> LQIYPQRRVIGHRIEIFRGKHRRRRMVPPRIPLHPLAANTSEETASKDMNLFETYRDLQLRWKKTCRQRKKKFNIARKWRMPRNIRPLPDPSWTLVFHVNPRSGYRRGRGVCRDRRRENLQGDALEVSAEDEENRLAGKAPSNRDQEDRQRGRGAQETYFRSGAALDAAIEEENILQIL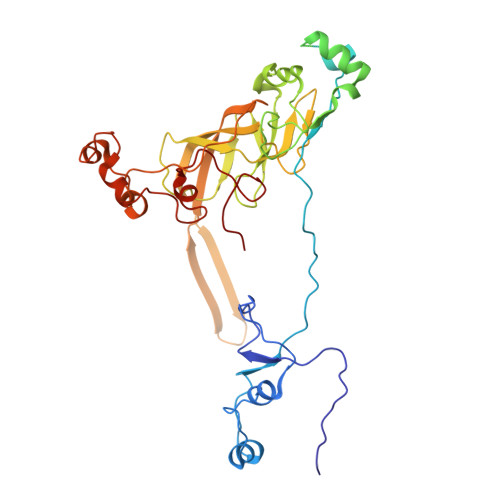ARHPEKGRVEGSGRPRGADGWGRDGPLPQWMQILQRTPQEELFCVMKSNVSTQHKVTAGDLIQAEKLHRKQAGDKVVFGTVMLVGSRDWTIIGKPTVPFAKVEATVEEQTLAGETLSFFYRKSRRVSRFRRIRHCVTMLRIDRIVVDPNMTVDPPAPKPDRLLDLWANRWLYPDELDGIKRNESGEPVVSEIYDGREHQKGSYQRRGLTASYRWYPDPQSAHWRP D,L-endopeptidase RipA is the major PG hydrolase required for daughter cell separation in Mycobacterium tuberculosis ( Mtb ), as RipA defects severely hinder cell division and increase antibiotic vulnerability. Despite extensive studies, the mechanisms governing Mtb RipA regulation remain controversial and poorly understood. Here, we report an integrative structural and functional analysis of the SteAB system, a regulatory complex that has been shown to modulate cell separation in the model organism Corynebacterium glutamicum ( Cglu ) and is conserved across Mycobacteriales .

In addition, crystallographic characterization of the cytoplasmic core of SteA revealed a homodimeric organization harboring a conserved functional pocket similar to the phosphonucleotide-binding site of thiamine pyrophosphokinase. These data, coupled with the in vivo phenotypic analysis of a steAB knockout mutant of Cglu , support a model in which the transmembrane SteAB heterotetramer, driven by cytoplasmic ligand binding, orchestrates the productive periplasmic positioning of RipA, leading to PG hydrolysis activation.

>[8x]DLPGLQGATRICTPQGKGLKRLSEGDLAIIDAPDLSRTFAQRLLAAKPAAVLNVSRFTTGSVPNFGPQMLIDGGIQLVEGFGQELLDGTKDGKKGRLTEDGQLFYGERLISNGSVLSGPAAENAFADAQQSLLDRMEAYFGNTIQFIHSEAPLLIDGLGIPDTGNAIEGRKVLIASPGDNHRSRLKELRSFIREYDPVLIGVDGAADTLVELGYKPALIVGNPTGIGADALRSGANVILPADPDGHAVGLERIQDLGIGAMTFPSSVNSSTDLALLLADFHNPQMIVNVGGPVTLDGVFENREDSDPAALLTRAKLGTKLVDGSVIASLYTVR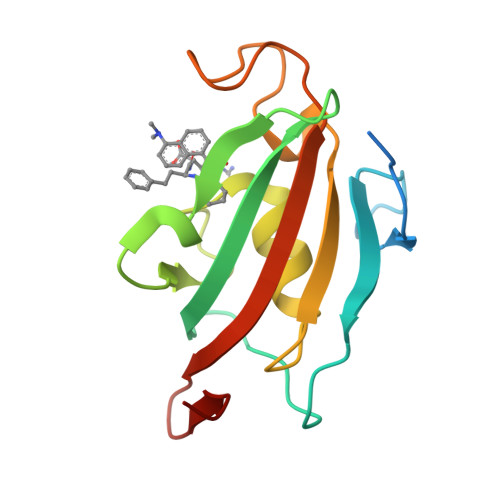> MTAEEMKATESGAQSAPLPMEGVDISPKQDEGVLKVIKREGTGTEMPMIGDRVFVHYTGWLLDGTKFDSSLDRKDKFSFDLGKGEVIKAWDIAIATMKVGEVCHITCKPEYAYGSAGSPPKIPPNATLVFEVELFEFKGEDLTEEEDG>SMSRFAADPHWLIYLPPTMSPCETSKKEGMLEHPIEAFEYFRTRGVGKVVCEQKHMGSRAVVIVCKDSQVAEKRFGVLDGTAGICYTRTGRHFFDDMQLEAELIDRVRKVLDKSGFWGDFNTDWVCLDCELMPWSAKAQKLLEEQYSAVGISGRVVLDEAVKLLKQASLNKTVSFDVSRQTSGKNADINELLQRFTERSEMMQKYVEAYRKYCWPVNSIDDLKLAPFHILATEGKVHSDKNHIWHMDTIAKYCTQDDSLIMATNHILVDVTDAESVDKGIKWW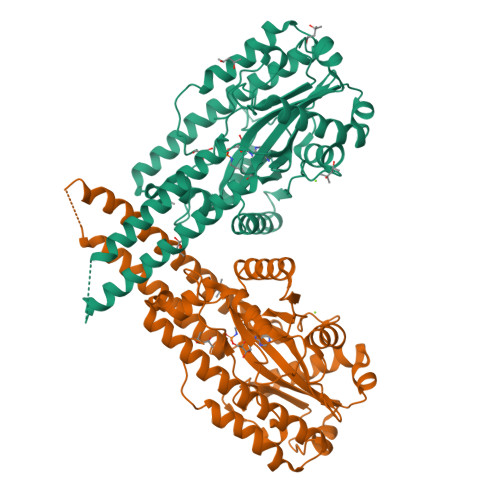EDLTASGGEGMVVKPYDFIVKNGRELLQPAVKCRGREYLRIIYGPEYTMDENIERLRNRAVGKKRSLALREFSLGMEALERFVRNEPLYRVHECVFGVLALESEPVDPRL[4x]>TTGHSYEKYNNWETIEAWTKQVTSENPDLISRTAIGTTFLGNNIYLLKVGKPGPNKPAIFMDCGFHAREWISHAFCQWFVREAVLTYGYESHMTEFLNKLDFYVLPVLNIDGYIYTWTKNRMWRKTRSTNAGTTCIGTDPNRNFDAGWCTTGASTDPCDETYCGSAAESEKETKALADFIRNNLSSIKAYLTIHSYSQMILYPYSYDYKLPENNAELNNLAKAAVKELATLYGTKYTYGPGATTIYPAAGGSDDWAYDQGIKYSFTFELRDKGRYGFILPESQI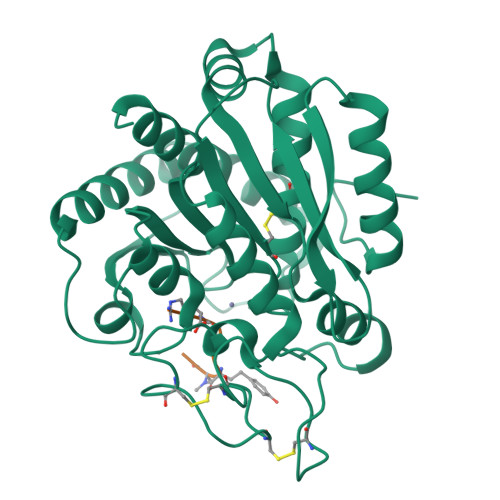QATCEETMLAIKYVTNYVLGHL[3x];>RKVYAF[3x]>DVIYYYQGQITVGNVAPPMYFAIQPNGNAKIGNNSNVPSYINAQPSSGGSGFTAQVNITNATYNYYFNFMGLAVSKTGYIYLAKVAYSYTATNNPIQNATLYIMNQQGQIVYKYKLIVNGVVNSTLPSTPLQINSGSYIVSLLIVPYQGTLPKTPSNDLATITVNFGFSPMTASPPPIPLPSP[5x]

While some archaea produce only one type of filament, the archaeal model species Sulfolobus acidocaldarius generates four. These include rotary swimming propellers analogous to bacterial flagella (archaella), pili for twitching motility (Aap), adhesive fibres (threads), and filaments facilitating homologous recombination upon UV stress (UV pili). Here, we use cryo-electron microscopy to describe the structure of the S. acidocaldarius archaellum at 2.0 Å resolution, and update the structures of the thread and the Aap pilus at 2.7 Å and 2.6 Å resolution, respectively. We define distinct N-glycan patterns in the three filaments and identify a putative O-glycosylation site in the thread.

Through cryoEM and visual proteomics, we previously determined that the thread consists of multiple copies of the subunit Saci_0406, and resembles, but is not homologous to, bacterial Type-I (chaperone-usher; CU) pili. Saci_0406 consists of a β-strand rich globular c-terminus and an extended N-terminal β-strand. Like in CU pili, the N-terminal strand inserts into a downstream subunit, thereby completing a β-sheet via donor strand complementation (DSC). The subunits additionally form intermolecular isopeptide bonds, thus covalently interlinking the thread into a strong, chain-like fibre. To facilitate this analyis, we improved the resolution of the structures of the thread and Aap from the previously published resolutions of 3.5 Å15 and 3.2 Å9, to 2.7 Å and 2.6 Å, respectively. Owing to its distinct architecture, the thread is considerably thinner (40 Å) than archaella (110 Å) and Aap (80 Å). Our new 2.7 Å resolution cryoEM map of the thread reveals a putative O-glycan modification at residue T195. We were able to model a mannose molecule into the density, with α-mannose resulting in a better fit than β-mannose. The finding of the putative O-glycan is surprising, as so far, no O-glycosylation has been reported in any other experimentally solved surface structure of S. acidocaldarius. To address this question, we modelled archaella, Aap and threads through the pores of the S. acidocaldarius S-layer. This revealed that the threads are thin enough to traverse the hexagonal pores.1H-indol-6-ol | C8 H7 N O | 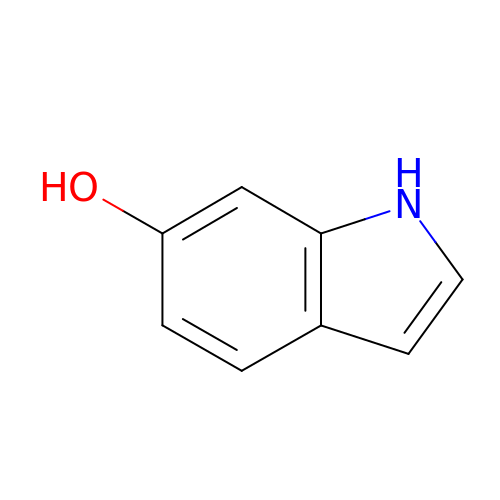XAWPKHNOFIWWNZ-UHFFFAOYSA-N> GSHMGLGGGGGGEGEEGSGGETTPPEGNYTTAKWQPAVGTKWQIELLYALNDTSVDAEIYDIDLFINDKSTIAGLQRAGRKVICYFSAGSYENWRPDKDKFKDSDLGHD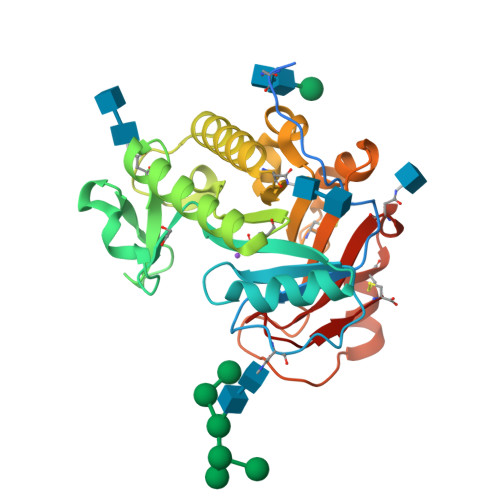LDDWPGEKWLNISSANVRQIMLDRLDMARDKGCDGVDPDNVDGYDNDNGLDLTQADSISFVNFLANAAHARNMSIGLKNAGDIIPSVIKNMQWSVNEQCAQYNECDTYAVFPQNGKPVFHIEYPKGDKTNNDLSVTASQKNAACDFAGSANFSTVIKNMNLNNWVEYC> PPAR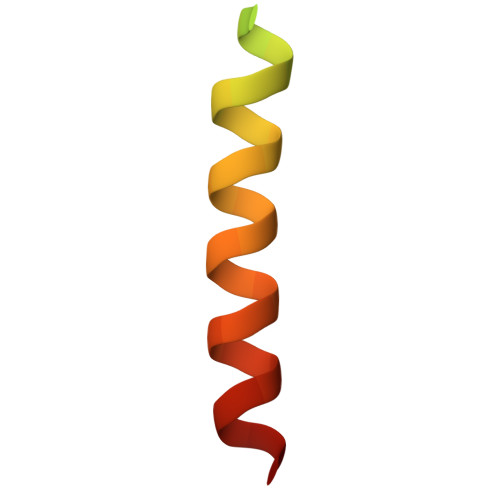KEKTKVKESVSRVEKAKQKSAQQELKQRQRAEIYALNRVMTE> MRKRVVVTGVGAIHPDGNDVTAIKSKVIQKLLGQESKNNTTASSIIRTLSDFDGAKYINNRLRRKIDEFSVYGIVAVEMALKASRLDVDKLDPNRVGIYVGNCFGGWQHIEDEVKALHIEGIKGMGPYVATAWFPAALQGQLSLLYGFSAQS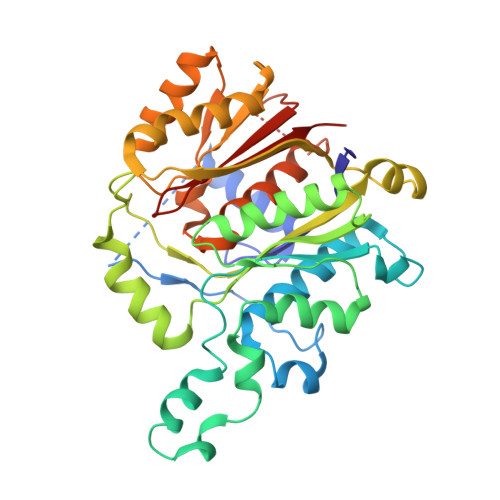KTFSTSDVAGMQAIGYAAEAISNGVAEVMLCGASEHLSSPLVKNLLEKTSSQKHSEVFGEKQPGDFSEGAAFLVLEERQHALERGASILCELTGFVDYFAPDKNTRNNTLEYTAELFNHNENAVFIMDGIYDDEKEITSKAFSNKEIKTSFINLRPYLDNQFSVSGVIDSVLASSFLSESHGDEEQQSKKINEFSNTNQIIIQRFSNQGHVCALSFSAI3'-O-[(R)-{[(2R,3aR,4R,6R,6aR)-6-(2-amino-6-oxo-1,6-dihydro-9H-purin-9-yl)-2-hydroxy-2-oxidotetrahydrofuro[3,4-d][1,3,2]dioxaphosphol-4-yl]methoxy}(hydroxy)phosphoryl]uridine 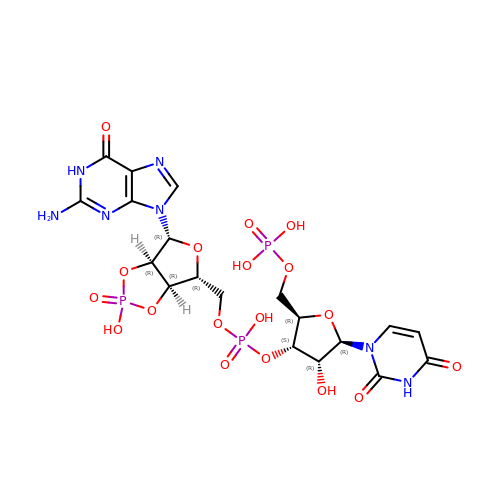5'-(dihydrogen phosphate) | C19 H24 N7 O18 P3 | UIVVUPHFWRPLKC-VMIOUTBZSA-N> KWYYKTITFLPELCNNESLAAKCLRVLHGFNYQYETRNIGVSFPLWCDATVGKKISFVSKNKIELDLLLKQHYFVQMEQLQYFHIS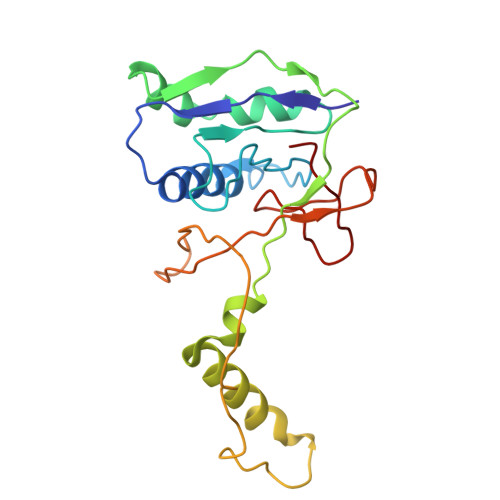NTVLVPEDCTYVSFRRCQSIDKLTAAGLARKIRRLEKRALSRGEAFDPSSFAQKEHTAIAHYHSLGESSKQTNRNFRLNIRMLSEQPREGNSIFSSYGLANSENSFQPVPLI>[2x]MSLRSHFATQKDQWQTYTKEKKIKIGFDATFVPMGYEEKDGSYIGFDIDLANAVFKLYGIDVEWQAIDWDMKETELKNGTIDLIWNGYSVT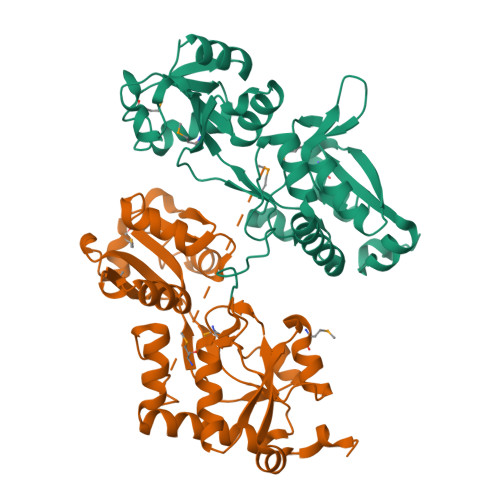DERKQSADFTEPYMVNEQVLVTKKSSGIDSVAGMAGKTLGAQAGSSGYDAFNASPKILKDVVANQKVVQYSTFTQALIDLNSGRIDGLLIDRVYANYYLEKSGVLDQYNVMPAGYEGESFAVGARKVDKTLIKKINQGFETLYKNGEFQKISNKWFGEDVATDQVKGKREGHHHHHH The faithful and efficient copying of chromosomal DNA is performed by chromosomal replicases, which generate double-stranded DNA from primed, single-stranded DNA. These replicases achieve great speed and processivity by tethering to ring-shaped protein complexes called sliding clamps, which encircle DNA and have the ability to slide freely along the DNA strand. In E. coli, the sliding clamp is the β subunit of the pol III holoenzyme (β clamp), and the eukaryotic sliding clamp is called Proliferating Cell Nuclear Antigen (PCNA). The sliding clamps share a domain architecture that has a six-fold pseudosymmetric rotation axis running through the center of the clamp and a central pore lined with α-helices through which DNA is threaded. The central hole within the sliding clamp is lined with α-helices that present a number of conserved, positively charged residues, creating a surface that complements the negatively charged DNA backbone.

To overcome this problem, we generated a single-chain construct of PCNA in which three PCNA monomers are fused together by two 11-residue linkers (specified in Methods). In an attempt to crystallographically trap an open clamp, the single-chain PCNA contained mutations R110S and Y114S in the first subunit. The PCNA in the model is very well resolved and, despite these mutations, is closed and does not significantly deviate from wild-type PCNA. We used one of these datasets for the analysis presented here, derived from a crystal that incorporated a 10-base pair DNA construct with a four-base 5' overhang on one end. Based on this weak density, we placed a 10-base pair B-form DNA in the center of the PCNA ring at a tilt of ~40° with respect to the rotation axis of PCNA. Refinement of coordinates and temperature (B) factors for individual atoms in this PCNA-DNA model resulted in very high temperature factors for the atoms in the DNA (in the range of about 125-450 Å2). This indicates that the DNA is partially disordered or has low occupancy, and the resolution of the dataset does not permit reliable refinement of individual atomic positions for the DNA. Inspection of the position of the partially disordered DNA in our model reveals potential interactions between DNA and the center of PCNA. The most extensive type of PCNA-DNA interaction occurs on DNA strand 1; a number of positively charged residues that reside on the helices lining the center of PCNA, especially Lys 13, Arg 14, Lys 146, and Arg 149 of subunit A and Lys 146 and Arg 149 of subunit C, create a surface that complements the negatively charged phosphate oxygens of bases 1 to 5 (see numbering, Figures 6A &6D). A second loop, which extends from the lower portion of the central pore of PCNA and presents the sidechains of Asn 83 and Asn 84 towards the DNA, makes contact with DNA strand 1 from two different subunits; from subunit A to the phosphate group of base 2, and from subunit B to the phosphate groups of bases 6 and 7.

> GPHMASMLEAKFEEASLFKRIIDGFKDCVQLVNFQCKEDGIIAQAVDDSRVLLVSLEIGVEAFQEYRCDHPVTLGMDLTSLSKILRCGNNTDTLTLIADNTPDSIILLFEDTKKDRIAEYSLKLMDIDADFLKIEELQYDSTLSLPSSEFSKIVRDLSQLSDSINIMITKETIKFVADGDIGSGSVIIKPFVDMEHPETSIKLEMDQPVDLTFGAKYLLDIIKGSSLSDRVGIRLSSEAPALFQFDLKSGFLQFFLAPKFNDEGSNSQSNGSGALEAKFEEASLFKRIIDGFKDCVQLVNFQCKEDGIIAQAVDDSRVLLVSLEIGVEAFQEYRCDHPVTLGMDLTSLSKILRCGNNTDTLTLIADNTPDSIILLFEDTKKDRIAEYSLKLMDIDADFLKIEELQYDSTLSLPSSEFSKIVRDLSQLSDSINIMITKETIKFVADGDIGSGSVIIKPFVDMEHPETSIKLEMDQPVDLTFGAKYLLDIIKGSSLSDRVGIRLSSEAPALFQFDLKSGFLQFFLAPKFNDEGSNSQASNSGALEAKFEEASLFKRIIDGFKDCVQLVNFQCKEDGIIAQAVDDSRVLLVSLEIGVEAFQEYRCDHPVTLGMDLTSLSKILRCGNNTDTLTLIADNTPDSIILLFEDTKKDRIAEYSLKLMDIDADFLKIEELQYDSTLSLPSSEFSKIVRDLSQLSDSINIMITKETIKFVADGDIGSGSVIIKPFVDMEHPETSIKLEMDQPVDLTFGAKYLLDIIKGSSLSDRVGIRLSSEAPALFQFDLKSGFLQFFLAPKFNDEE> MFNQPPRFQNYFFQSYLLIYENTPVGSSITQLTAVDPDGEPLIFGVVGEEASRFFAVQENTGVVWLRQPLDRETKSEMQVVFSVSDSQGVVKDTVNIQIGDVNDNAPTFHNQPYTVNIPEDTSVGTSIFMVNATDPDQ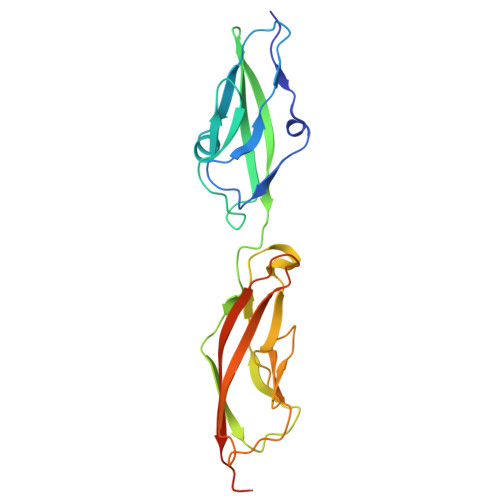GTGGSVLFSFQPPSPFFSIDGARGIITVSRLLDYEVTSAYQLTVNATDQDKLHPLSSLANLAITLSDIQDRDLEHHHHHH ethyl 1-(cyclopentylmethyl)-5-pyridin-4-yl-indole-2-carboxylate 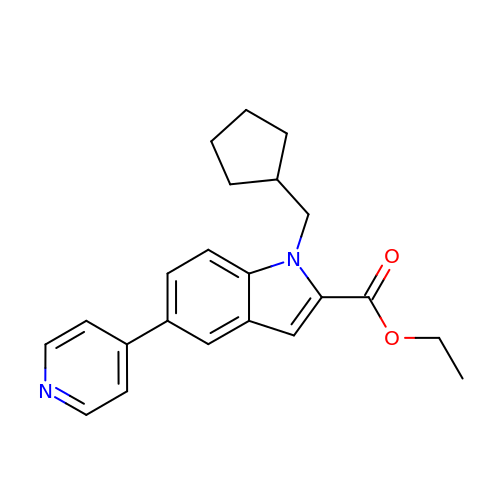| C22 H24 N2 O2 | XLAIBBWMNVOQSY-UHFFFAOYSA-N> KEPCPPENLQLTPRALVGKWYLRTTSPDIFKQVSNITEFYSAHGNDYYGTVTDYSPEYGLEAHRVNLTVSGRTLKFYMNDTHEYDSKYEILAVDKDYFIFYGHPPAAPSGLALIHYRQSCPKEDVIKRVKKALKNVCLDYKYFGNDTSVPCHYVE

Diploptera punctata, also known as the Pacific beetle cockroach, is a viviparous cockroach that gives birth to live offspring and secretes a highly concentrated mixture of glycosylated proteins as a source of nourishment for developing embryos. The principal component of this milk is lipocalin-like proteins or Lili-Mips. Lili-Mip has a lipocalin fold and binds to different fatty acids and other moieties. Lili-Mip is small (18.8 kDa), monomeric, and glycosylated.

The intrinsic tryptophan fluorescence change was employed to determine the binding affinity of different fatty acids to Lili-Mip1. Fatty acids of varying chain lengths (14, 16, and 18) and degrees of unsaturation (0, 1, and 2) were assayed. All tested fatty acids bound with micromolar range affinities to the different Lili-Mips. Binding studies with Lili-Mip1 against palmitic acid were performed at different pH values to verify whether the fatty acid binding affinity was pH-dependent. The data showed that Lili-Mip1 had no change in binding affinity for palmitic acid between pH 4.8 and 8.2(KD’s at pH 4.8, 7.2, and 8.2 for Palmitic acid are 1.76± 0.93; 0.44±0.20; 2.24±0.11 μM respectively). Deglycosylated Lili-Mip1 showed a marginal decrease in stability. However, the removal of glycans did not affect the pH-dependent change in the thermal stability of Lili-Mip1. In various crystal structures (reported here and previously by us), Phe-98 and Phe-100 occupy multiple conformations in the binding pocket. Here we show Phe-98 and Phe-100 can reorient to stabilize interactions at the bottom of the cavity–and change the volume of the cavity from 510 Å3 to 337 Å3. The different conformations of Phe-98 and Phe-100 allow Lili-Mips to bind fatty acids of different lengths, thereby explaining the broad substrate tolerance of Lili-Mips.> MKLQKQLLEAVEHKQLRPLDVQFALTVAGDEHPAVTLAAALLSHDAGEGHVCLPLSRLENNEASHPLLATCVSEIGELQNWEECLLASQAVSRGDEPTP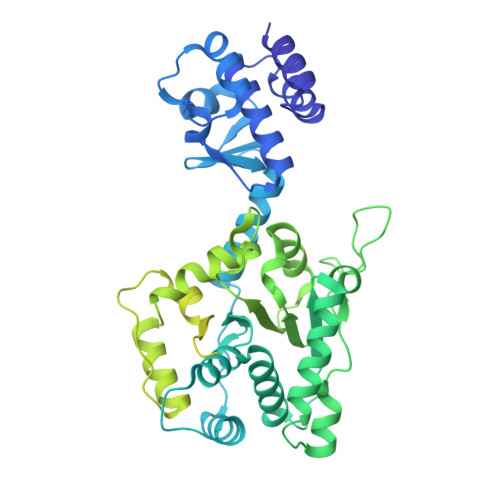MILCGDRLYLNRMWCNERTVARFFNEVNHAIEVDEALLAQTLDKLFPVSDEINWQKVAAAVALTRRISVISGGPGTGKTTTVAKLLAALIQMADGERCRIRLAAPTGKAAARLTESLGKALRQLPLTDEQKKRIPEDASTLHRLLGAQPGSQRLRHHAGNPLHLDVLVVDEASMIDLPMMSRLIDALPDHARVIFLGDRDQLASVEAGAVLGDICAYANAGFTAERARQLSRLTGTHVPAGTGTEAASLRDSLCLLQKSYRFGSDSGIGQLAAAINRGDKTAVKTVFQQDFTDIEKRLLQSGEDYIAMLEEALAGYGRYLDLLQARAEPDLIIQAFNEYQLLCALREGPFGVAGLNERIEQFMQQKRKIHRHPHSRWYEGRPVMIARNDSALGLFNGDIGIALDRGQGTRVWFAMPDGNIKSVQPSRLPEHETTWAMTVHKSQGSEFDHAALILPSQRTPVVTRELVYTAVTRARRRLSLYADERILSAAIATRTERRSGLAALFSSRE>UGCGGGGUC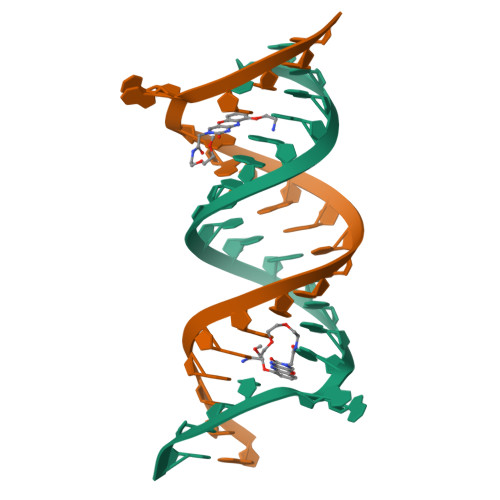CCGGGAGGACCGC[2x]> MSNGDWGQSQRTRGTGPVRGIRTMDVNAPGGGSGGSALRILGTASCNQAHCKFGRFAGIQCVSNCVLYLVKSFLAGRPLTSRPELDEVLDEGARLDALMRQSGILKGHEMAQLTDVPSSVVLRGGGRVHIYRSAEIFGLVLFPAQIANSAVVQSLAEVLHGSYNGVAQFILYICDIYAGAIIIETDGSFYLFDPHCQKDAAPGTPAHVRVSTYAHDILQYVGAPGAQYTCVHLYFLPEAFETEDPRIFMLEHYGVYDFYEANGSGFDLVGPELVSSDGEAAGTPGADSSPPVMLPFERRIIPYNLRPLPSRSFTSDSFPAARYSPAKTNSPPSSPASAAPASAAPASAAPASAAPASAAPASAAPASAAPASAAPASSPPLFIPIPGLGHTPGVPAPSTPPRASSGAAPQTPKRKKGLGKDSPHKKPTSGRRLPLSSTTDTEDDQLPRTHVPPHRPPSAARLPPPVIPIPHQSPPASPTPHPAPVSTIAPSVTPSPRLPLQIPIPLPQAAPSNPKIPLTTPSPSPTAAAAPTTTTLSPPPTQQQPPQSAAPAPSPLLPQQQPTPSAAPAPSPLLPQQQPPPSAARAPSPLPPQQQPLPSATPAPPPAQQLPPSATTLEPEKNHPPAADRAGTEISPSPPFGQQPSFGDDASGGSGLVRYLSDLEEPFLSMSDSEEAESDLASDIPTTEDEDMFEDEVFSNSLESGSSAPTSPITLDTARSQYYQTTFDIETPEMDFVPLESNIARIAGHTYQEQAIVYDPASNREVPEADALSMIDYLLVTVVLEQGLIRSRDRSSVLNLLEFLKDWSGHLQVPTLDLEQLLTSELNIQNLANMLSENKGRAGEFHKHLAAKLEACLPSLATKDAVRVDAGAKMLAEIPQLAESDDGKFDLEAARRRLTDLLSGGDQEAGEGGGEPEDNSIYRGPHVDVPLVLDDESWKRLLSLAEAARTAVARQQAGVDEEDVRFLALLTAIEYGAPPAASVPPFVHNVAVRSKNAALHVRRCTADIRDKVASAASDYLSYLEDPSLPTVMDFDDLLTHLRHTCQIIASLPLLNIRYTSIEWDYRELLYLGTALSDMSGIPWPLERVEEDDPSIAPLPEFETVAKKQKELETTRENEKRLRTILDDIEAMLGLAGVASAPGAPISPASPSATPANHDNPEATPPLADTAALTIPVIEKYIANAGSIVGAAKNPTYIRLRDTIQQIVRSKKYLMNILKSITFYTIDNYIASFEESIDHLYRDLPVLDPEVQDGIDRILDPMVSEALHTFEMGNRLTLEPARLVALQNFATHSTLKETAAAVNLLPGLLAVYDATITGQAPEDALRLLSGLQNQLSQTLIPGKLKKRFLSYLQKLKNNNNDQLRQKEVQAWRLEAEGFKPATEEQLEAFLDTAPNKELKRQYEKKLRQLMETGRKEKEKLREQEDKERQERRAREANEAWARIRKALGARPEPAPTSPDDWNTLLASLLPDNTDSAAAAAAAVARNTDILDSLTQILAAMLLGITRVRRERLRSLLVDDGGAAERMEAAEPGWFTDIETGPLARLDAWPATPAATAKEGGGGRGAEEAAGALFRARTAADAIRSALAQTRQALQSPDMKSAVVNTDLEAPYAEYERGLAGLLEKRRAAEAALTAIVSEYVDRTLPEATNDPGQANLPPPPTIPQATAPPRLASDSALWPKKPQLLTRRERDDLLQATGDFFSELLTEAEAAEVRALEEQVRESQTLMAKAHEMAASTRRGFHTALEAVLSRSRDEAPDDELRSLLPSPPKAPVQAPLEAALARAAAGNGSWPYRKSLAAAKWIRGICEAVRGLSEGALALAGGAGAWLNLAAAADGEIHELTRLLEVEGMAQNSMDGMEELRLALATLDPKRVAGGKETVADWKRRLSRLEAIIQEAQEESQLQGTLQDLVTQARGHTDPRQLKIVVEAARGLALGASAGSQYALLKDKLLRYASAKQSFLAFYETAQPTVFVKHPLTNNLPLLITISAPPTGWGNGAPTRRAQFLAAAGPAKYAGTLWLETESPCDPLNPAYVSADTQEPLNYIPVYHNFLEYVMPTVLENPEAFSLTPAGRPQAIGPPQDDQERRRRTLASVASARLSAAAADSYWDTWPDVESNAGELLREYVSAPKALMEDLADNPIVAMTLLAHASLIASRNHPPYPAPATDREVILLEQREMMALLVGTHPAYAAAFLGAPSFYAGLGLVSALARDGGLGD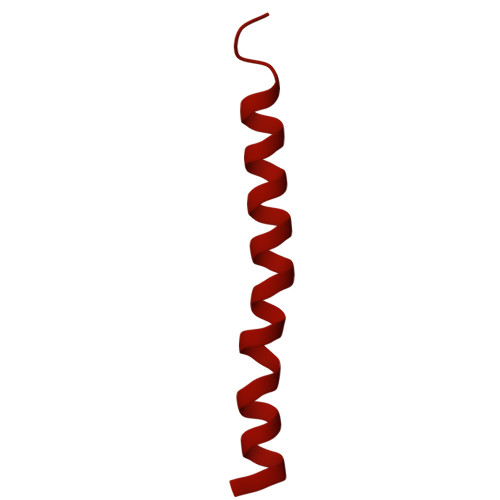LLSDSVLTYRLVRSPASGRGGMPSTTRGSNDGEDARRLTRHRIAGPPTGFIFFQDAWEEMDTRAALWPHPEFLGLVHNQSTARARACMLLLARRCFAPEALQQLWHSLRPLEGPVAFQDYLRDFVKQAYTRGEELPRAEGLEVPRETPSSYGTVTGRALRNLMPYGTPITGPKRGSGDTIPVSVFEAAVAAAFLGRPLTLFVSSQYLFNLKTLGQVRVVAPLLYCDGHSEPFRSLVETISLNFLQDLDGYSESFEPEMSIFARQAVWLRELLTEARAAKPKEARPPTVAILANRKNIIWKCFTYRHNLPDVQFYFNAAGASRWPTDVLNPSFYEHEDPPLPVGYQLPPNPRNVQELFSGFPPRVGHGLVSGDGFQSADNTPASSDRLQQLGGGETDQGEKGSTTAESEASGPPSPQSPLLEKVAPGRPRDWLSPTSSPRDVTVTPGLAAPITLPGPRLMARPYFGAETRASESPDRSPGSSPRPWPKDSLELLPQPAPQQPPSSPWASEQGPIVYTLSPHSTPSTASGSQKKHTIQIPGLVPSQKPSYPPSAPYKPGQSTGGIAPTPSAASLTTFGLQPQDTQASSQDPPYGHSIMQREKKQQGGREEAAEIRPSATRLPTAVGLRPRAPVVAAGAAASATPAFDPGEAPSGFPIPQAPALGSGLAAPAHTPVGALAPRPQKTQAQRPQDAAALPTPTIKAVGARPVPKATGALAAGARPRGQPTAAPPSAASPPRVSLPVRSRQQQSPAIPLPPMHSGSEPGARPEVRLSQYRHAGPQTYTVRKEAPPSAASQLPKMPKCKDSMYYPPSGSARYPAPFQALSFSQSVASPAPSSDQTTLLWNTPSVVTQFLSIEDIIREVVTGGSTSGDLVVPSGSPSSLSTAAPEQDLRYSLTLSQASRVLSRFVSQLRRKLERSTHRLIADLERLKFLYL> MATNQQLSIALRIQADLAEAQNALRQLTGNLQQVDRGAVQTRSELSAMGGQLDSLRAQVLGFVGAWASLSALGGLVTMVDQYGQMADRIQMVTSSTAEYEQVQARLLETASRTYRPLAEAQELYIRTADSLKSLRYTTEQALDITDSFSFLLVTNAASADRAASAIDAYSKSIQTGKVSSDAWQSIMAAMPSLVNALAESTGKSTEEIRKLGIEGSLSLRDLNEGLRKTVAANREAADNMGTSVQDALVSLNNALSAYLGELNRTYDITGSVSSALNVLAENMEVIVKLFGVAAVAGLTRYVASLTLATQAKLAAVLAARAQAAEELRTAQAQVASTAAAAANARAQAGLTVSHTQAAAAEAAHTAATQRLAAAQLAAGAAMRGMLAVIGGPAGIAMLVAGAAASFFLFRDSAQAVKSSLDDLSEPLDQVVERMGKLSEIEQDRELTRLS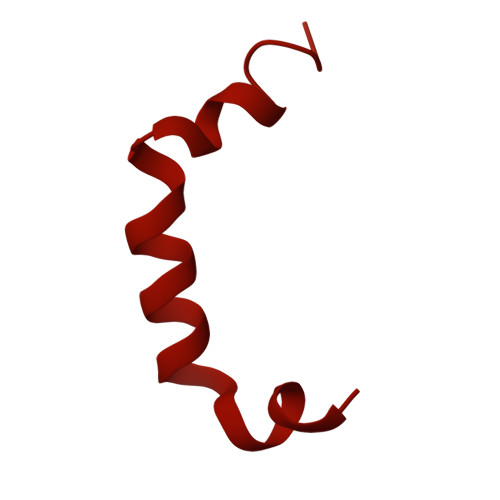EQIDGLRQTAVEAAREMREVASTALYGARLDRIPSAEAQQALQPLIDASADAARGVEVDWKSVMDTLAASGAVPDSLKRKLLDMAAGQAEAGRTATELGQRHAELKARLEGSTAAINENSDALSKGSDKAAEYIQSLRLAIADLEDPSVLGKAGRRLQQFGADLNAEQSAEILRLETLKANTEKAAQAREDARRKAESSARQQASTAEQLAKSQEGYVAGLEKQARTLGLTSAEVRAYELAEKGLTGALHARAAAALAALAADEKKRQADANARTNAGLEAEYLRATGRTVDAGLLEIRTKFDAMRRDFEKAGNDAGLAWIDKLIPVAEAKVRLDDVKQQMDDLLADQQRAESSVNVQQDAGVINEMDARQRILDIHRATYEKLQQIRPILEQMARQPGEVGRAAAESLAQLDAEAARLQQTTTLLETTLRDGLTTGFTDAIKGLASGTMDLRDAITSLGEAVLNALVNMAAQNLAQSLSSGIMGLFGGGQQDTSMTTGAAAVTASAGALSTAGASLLTGAAAIQAAAASLAAANGVQGLGAAAGGAGAAGAAAGGGSWLSSIAGIFGFASGGHIKGPGTGTSDSIPILASNDEFMTRAAVVRQPGALAFLEQFNRYGMAALAGWANPVRHATGGQIGTPAPNLPAPVRAGANLPEPSKNFSTSVANSIYLHAVQDTDQMAADMWAGKGGEHFLVWLNKNRQAVKQII The Saccharomyces cerevisiae B-family replicative DNA polymerases, namely Pol ϵ, Pol δ and Pol α, have been estimated to incorporate about 13 000 NTPs during each cell cycle of the yeast genome, and Pol ϵ seems to incorporate the majority of NTPs, roughly four times as many ribonucleotides as Pol δ. Other examples where an amino acid adjacent to the steric gate residue influences ribonucleotide discrimination are found among B-family polymerases. It was first shown in the ϕ29 DNA polymerase that B-family polymerases have a conserved tyrosine (Y645 in Pol ϵ) that functions as a steric gate. Our data show that Pol ϵ discriminates NTPs through the concerted action of a steric gate residue (Y645) and a sensor in the finger domain (N828). A comparison with other B-family DNA polymerases showed that both Y645 and N828 are structurally conserved residues, thus reinforcing their functional importance.

To test the hypothesis that steric hindrance does not allow the finger domain to adopt a completely closed conformation when a ribonucleotide is bound to the active site, we replaced N828 with a valine, which is both less bulky and unable to form a hydrogen bond with the β-phosphate of the incoming nucleotide. Compared to both the wild-type Pol2CORE-dATP and N828VPol2CORE-dATP structures, the presence of a ribonucleotide in the N828VPol2CORE structure did not induce any significant structural changes to the residues surrounding the ribonucleotide. The activity of N828VPol ϵ was comparable to wild-type Pol ϵ and M644GPol ϵ. Biochemical and genetic studies showed that the N828VPol ϵ variant has an increased propensity to incorporate NTPs, suggesting that N828 functions as a sensor for discriminating against ribonucleotides.

> GGDPHMMFGKKKNNGGSSTARYSAGNKYNTLSNNYALSAQQLLNASKIDDIDSMMGFERYVPPQYNGRFDAKDIDQIPGRVGWLTNMHATLVSQETLSSGSNGGGNSNDGERVTTNQGISGVDFYFLDEEGGSFKSTVVYDPYFFIACNDESRVNDVEELVKKYLESCLKSLQIIRKEDLTMDNHLLGLQKTLIKLSFVNSNQLFEARKLLRPILQDNANNNVQRNIYNVAANGSEKVDAKHLIEDIREYDVPYHVRVSIDKDIRVGKWYKVTQQGFIEDTRKIAFADPVVMAFAIATTKPPLKFPDSAVDQIMMISYMIDGEGFLITNREIISEDIEDFEYTPKPEYPGFFTIFNENDEVALLQRFFEHIRDVRPTVISTFNGDFFDWPFIHNRSKIHGLDMFDEIGFAPDAEGEYKSSYCSHMDCFRWVKRDSYLPQGSQGLKAVTQSKLGYNPIELDPELMTPYAFEKPQHLSEYSVSDAVATYYLYMKYVHPFIFSLCTIIPLNPDETLRKGTGTLCEMLLMVQAYQHNILLPNKHTDPIERFYDGHLLESETYVGGHVESLEAGVFRSDLKNEFKIDPSAIDELLQELPEALKFSVEVENKSSVDKVTNFEEIKNQITQKLLELKENNIRNELPLIYHVDVASMYPNIMTTNRLQPDSIKAERDCASCDFNRPGKTCARKLKWAWRGEFFPSKMDEYNMIKRALQNETFPNKNKFSKKKVLTFDELSYADQVIHIKKRLTEYSRKVYHRVKVSEIVEREAIVCQRENPFYVDTVKSFRDRRYEFKGLAKTWKGNLSKIDPSDKHARDEAKKMIVLYDSLQLAHKVILVSFYGYVMRKGSRWYSMEMAGITCLTGATIIQMARALVERVGRPLELDTDGIWCILPKSFPETYFFTLENGKKLYLSYPCSMLNYRVHQKFTNHQYQELKDPLNYIYETHSENTIFFEVDGPYKAMILPSSKEEGKGIKKRYAVFNEDGSLAELKGFELKRRGELQLIKNFQSDIFKVFLEGDTLEGCYSAVASVCNRWLDVLDSHGLMLEDEDLVSLICENRSMSKTLKEYEGQKSTSITTARRLGDFLGEDMVKDKGLQCKYIISSKPFNAPVTERAIPVAIFSADIPIKRSFLRRWTLDPSLEDLDIRTIIDWGYYRERLGSAIQKIITIPAALQGVSNPVPRVEHPDWLKRKIAT>MAEAKVLSGAGLRGQVAGQT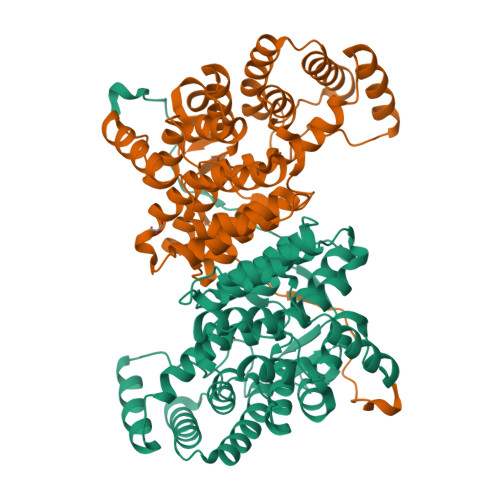ALSTVGQEGAGLTYRGYDVRDLAAAAIFEEVAYLLLYGELPNKQQLDAYLKKLQGQRDLPQALKEVLERIPKDAHPMDVMRTGASVLGTLEPELSFDQQRDVADRLLAAFPAIMTYWYRFTHEGQRIDCNSDEPTIGGHFLALLHGKKPSELHVKVMNVSLILYAEHEFNASTFTARVCASTLSDLYSCVTGAIGSLRGPLHGGANEAAMELIERFSSPQEATAELLKMLERKDKIMGFGHAIYKDSDPRNEVIKGWSKQLADEVGDKVLFAVSEAIDKTMWEQKKLFPNADFYHASAYHFMGIPTKLFTPIFVCSRTSGWTAHVFEQRANNRIIRPSAEYTGVEQRAFVPLEQR[4x]>[3x]MTDVQCEPALAGRKPKWADADIAELVDERTGRLDPRIYTDEALYEQELERIFGRSWLLMGHETQIPKAGDFMTNYMGEDPVMVVRQKNGEIRVFLNQCRHRGMRICRADGGNAKSFTCSYHGWAYDTGGNLVSVPFEEQAFPGLRKEDWGPLQARVETYKGLIFANWDADAPDLDTYLGEAKFYMDHMLDRTEAGTEAIPGIQKWVIPCNWKFAAEQFCSDMYHAGTTSHLSGILA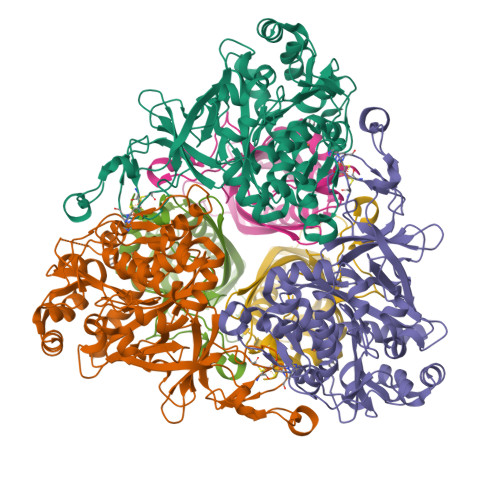GLPDGVDLSELAPPTEGIQYRATWGGHGSGFYIGDPNLLLAIMGPKVTEYWTQGPAAEKASERLGSTERGQQLMAQHMTIFPTCSFLPGINTIRAWHPRGPNEIEVWAFTVVDADAPEEMKEEYRQQTLRTFSAGGVFEQDDGENWVEIQQVLRGHKARSRPFNAEMGLGQTDSDNPDYPGTISYVYSEEAARGLYTQWVRMMTSPDWAALDATRPAVSESTHT;>[3x]MIDAESPTTAFRTKPAPVDPSLQHEIEQFYYWEAKLLNDRRFQEWFDLLAEDIHYFMPIRTTRIMRETAQEYSGAREYAHFDDNAQMMRGRLRKITSDVSWSENPASRTRHVISNVMIVDGEKPGEYHVSSVFIVYRNRLERQLDIFAGERKDILRRTGSEAGFELAKRTILIDQSTILSNNLSFFF(5R)-2-methyl-5-(prop-1-en-2-yl)cyclohex-2-en-1-one | C10 H14 O | 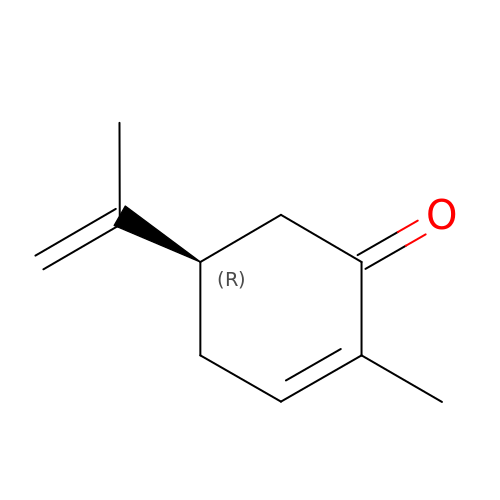ULDHMXUKGWMISQ-SECBINFHSA-N> GPLGSDLPPKVVPSKQLLHSDHMEMEPETMETKSVTDYFSKLHMG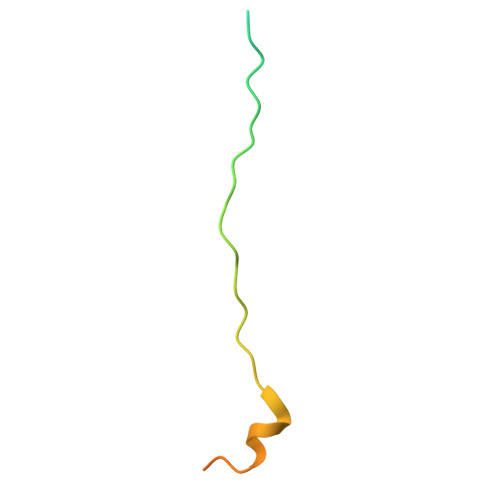SVAYSCTS> MGDSKVKVAVRVRPMNRREIDLHTKCVVDVEANKVILNPINTNLSKGDARGQPKIFAYDHCFWSMDESVREKCAGQDDVFKCLGENILQNAFDGYNACIFAYGQTGSGKSYTMMGTADQPGLIPRLCSGLFERTQKEENEEQSFKVEVSYMEIYNEKVRDLLDPKGSRQTLKVREHSVLGPYVDGLSKLAVTSYKDIE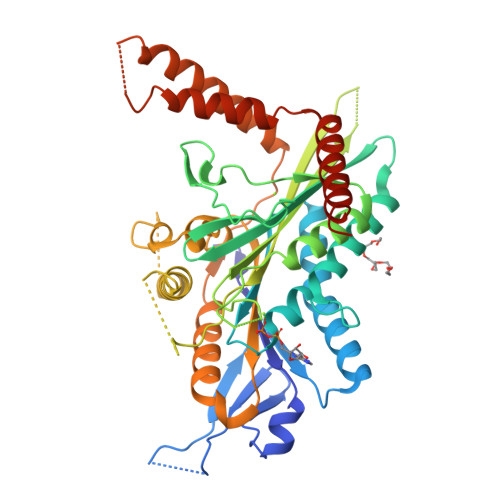SLMSEGNKSRTVAATNMNEESSRSHAVFKITLTHTLYDVKSGTSGEKVGKLSLVDLAGSERATKTGAAGDRLKEGSNINKSLTTLGLVISALADQGAGKNKNKFVPYRDSVLTWLLKDSLGGNSKTAMVATVSPAADNYDETLSTLRYADRAKHIINHAVVNEDPNARIIRDLREEVEKLREQLTKAEAMKSPELKDRLEESEKLIQEMTVTWEEKLRKTEEIAQERQKQLESHHHHHH>GFLTAFEYSEKRKMVFHITTGSQEFDKLLGGGIESMAITEAFGEFRTGKTQLSHTLCVTAQLPGAGGYPGGKIIFIDTENTFRPDRLR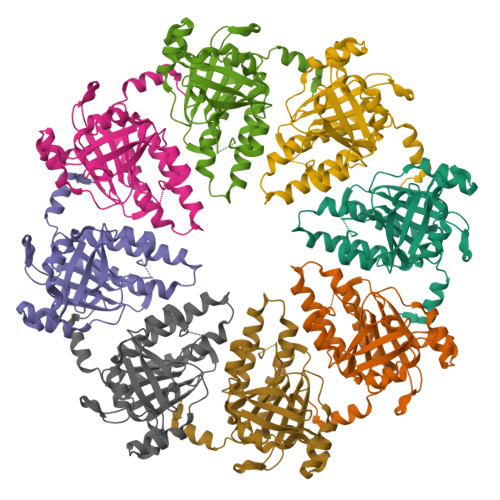DIADRFNVDHDAVLDNVLYARAYTSEHQMELLDYVAAKFHEEAGIFKLLIIDSIMALFRVDFSGRGELAERQQKLAQMLSRLQKISEEYNVAVFVTNQMTADPGATMTFQADPKKPIGGHILAHASTTRISLRKGRGELRIAKIYDSPEMPENEATFAITAGGIGDAKELEHHHHHH[4x]> AYDRAITVFSPDGRLFQVEYAREAVKKGSTALGMKFANGVLLISDKKVRSRLIEQNSIEAIQLIDDYVAAVTSGLVADARVLVDFARISAQQEKVTYGSLVNIENLVKRVADQMQQYTQYGGVRPYGVSLIFAG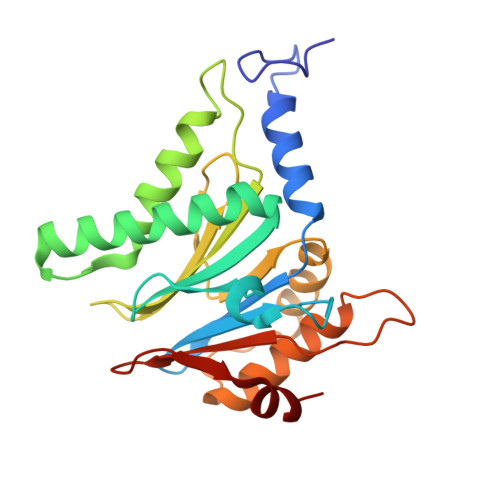IDQIGPRLFDCDPAGTINEYKATAIGSGKDAVVSFLEREYKENLPEKEAVTLGIKALKSSLEEGEELKAPEIASITVGNKYRIYDQEEVKKFL>[2x]MASMETSSSCESLGSQPAAARPPSVDSLSSASTSHSENSVHTKSASVVSSDSISTSADNFSPDLRVLRESNKLAEMEEPPLLPGENIKDMAKDVTYICPFTGAVRGTLTVTNYRLYFKSMERDPPFVLDASLGVINRVEKIGGASSRGENSYGLETVCKDIRNLRFAHKPEGRTRRSIFENLMKYAFPVSNNLPLFAFEYKEVFPENGWKLYDPLLEYRRQGIPNESWRITKINERYELCDTYPALLVVPANIPDEELKRVASFRSRGRIPVLSWIHPESQATITRCSQPMVGVSGKRSKEDEKYLQAIMDSNAQSHKIFIFDARPSVNAVANKAKGGGYESEDAYQNAELVFLDIHNIHVMRESLRKLKEIVYPNIEETHWLSNLESTHWLEHIKLILAGALRIADKVESGKTSVVVHSSDGWDRTAQLTSLAMLMLDGYYRTIRGFEVLVEKEWLSFGHRFQLRVGHG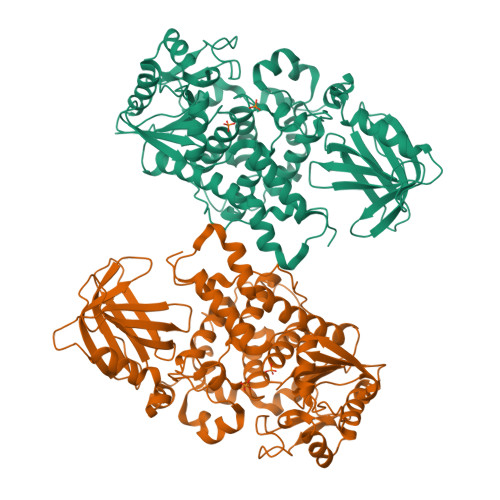DKNHADADRSPVFLQFIDCVWQMTRQFPTAFEFNEYFLITILDHLYSCLFGTFLCNSEQQRGKENLPKRTVSLWSYINSQLEDFTNPLYGSYSNHVLYPVASMRHLELWVGYYIRWNPRMKPQEPIHNRYKELLAKRAELQKKVEELQREISNRSTSSSERASSPAQCVTPVQTVVAAALEHHHHHH> MGSSLRPLYMDVQATTPLDPRVLDAMLPYLINYYGNPHSRTHAYGWESEAAMERARQQVASLIGADPREIIFTSGATESNNIAIKGVARFYRSRKKHLITTQTEHKCVLDSCRSLEAEGFQVTYLPVQKSGIIDLKELEAAIQPDTSLVSVMTVNNEIGVKQPIAEIGRICSSRKVYFHTDAAQAVGKIPLDVNDMKIDLMSISGHKIYGPKGVGAIYIRRRPRVRVEALQSGGGQERGMRSGTVPTPLVVGLGAACEVAQQEMEYDHKRISKLSERLIQNIMKSLPDVVMNGDPKHHYPGCINLSFAYVEGESLLMALKDVALSSGSACTSASLEPSYVLRAIGTDEDLAH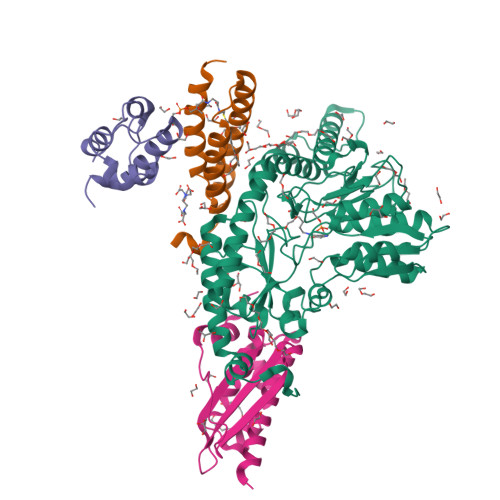SSIRFGIGRFTTEEEVDYTVEKCIQHVKRLREMSPLWEMVQDGIDLKSIKWTQH;> MAASSRAQVLALYRAMLRESKRFSAYNYRTYAVRRIRDAFRENKNVKDPVEIQTLVNKAKRDLGVIRRQVHIGQLYSTDKLIIENRDMPRT;> STIEERVKKIIGEQLGVKQEEVTNNASFVEDLGADSLDTVELVMALEEEFDTEIPDEEAEKITTVQAAIDYINGHQA;> MALHTQVVDHYENPRNVGSLDKTSKNVGTGLVGAPACGDVMKLQIQVDEKGKIVDARFKTFGCGSAIASSSLATEWVKGKTVEEALTIKNTDIAKELCLPPVKLHCSMLAEDAIKAALADYKLKQEPKKGEAEKKLEHHHHHH>[12x]MRGSHHHHHHGSLVPRGSMKKVSVIMPTFNNGEKLHRTISSVLNQTMKSTDYELIIIDDHSNDNGETLNVIKK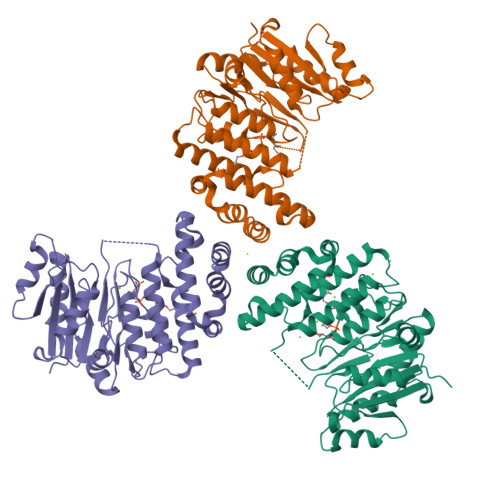YKGLVRFKQLKKNSGNASVPRNTGLKMSKAEYVFFLDSDDLLHERALEDLYNYGKENNSDLIIGKYGVEGKGRSVPKAIFEKGNVAKADIIDNSIFYALSVLKMFKKSVIDKNKIKFKTFSKTAEDQLFTIEFLMNSKNYSIKTDYEYYIVVNDFESSNHLSVNKSTGNQYFATINEIYKAIYKSPIYKNQEKRHQLAGKYTTRLLRHGQKKNFANSKMKYEDKIEWLNNFSKTINKVPRDSDKYVTQIFNLKLEAIRQNDLLAVMIADKLL> GASGDGAGASRQRKLEALIRDP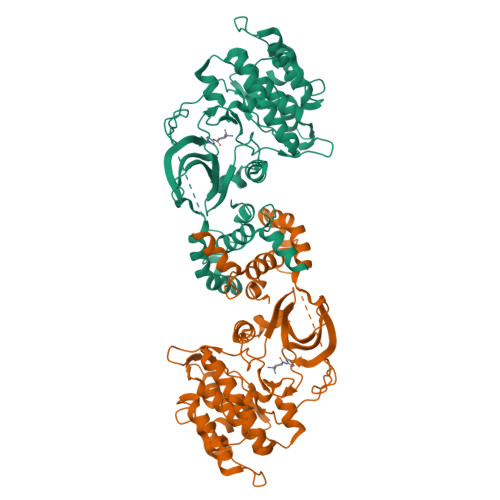RSPINVESLLDGLNSLVLDLDFPALRKNKNIDNFLNRYEKIVKKIRGLQMKAEDYDVVKVIGRGAFGEVQLVRHKASQKVYAMKLLSKFEMIKRSDSAFFWEERDIMAFANSPWVVQLFCAFQDDKYLYMVMEYMPGGDLVNLMSNYDVPEKWAKFYTAEVVLALDAIHSMGLIHRDVKPDNMLLDKHGHLKLADFGTCMKMDETGMVHCDTAVGTPDYISPEVLKSQGGDGYYGRECDWWSVGVFLFEMLVGDTPFYADSLVGTYSKIMDHKNSLCFPEDAEISKHAKNLICAFLTDREVRLGRNGVEEIKQHPFFKNDQWNWDNIRETAAPVVPELSSDIDSSNFDDIEDDKGDVETFPIPKAFVGNQLPFIGFTYYR> ATGC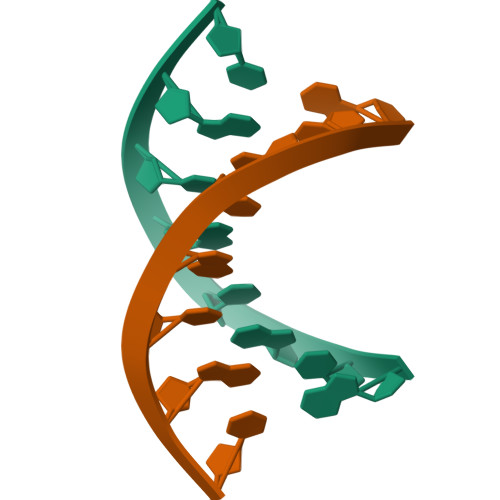GCAT>MELYRDPSQPIEVRVRDLLSRMTLEEKVAQLGSVWGYELIDERGKFSREKAKELLKNGIGQITRPGGSTNLEPQEAAELVNEIQRFLVEETRLGIPAMIHEECLTGYMGLGGTNFPQAIAMASTWDPDLIEKMTTAVREDMRKIGAHQGLAPVLDVARDPRWGRTEETFGESPYLVARMGVSYVKGLQGEDIKKGVVATVKHFAGYSASEGGKNWAPTNIPEREFKEVFLFPFEAAVKEANVLSVMNSYSEIDGVPCAANRKLLTDILRKDWGFEGIVVSDYFAVKVLEDYHRIARDKSEAARLALEAGIDVELPKTECYQYLKDLVEKGIISEALIDEAVTRVLRLKFMLGLFENPYVEVEKAKIESHRDIALEIARKSIILLKNDGILPLQKNKKVALIGPNAGEVRNLLGDYMYLAHIRALLDNIDDVFGNPQIPRENYERLKKSIEEHMKSIPSVLDAFKEEGIEFEYAKGCEVTGEDRSGFEEAIEIAKKSDVAIVVVGDKSGLTLDCTTGESRDMANLKLPGVQEELVLEVAKTGKPVVLVLITGRPYSLKNVVDKVNAILQVWLPGEAGGRAIVDIIYGKVNPSGKLPISFPRSAGQIPVFHYVKPSGGRSHWHGDYVDESTKPLFPFGHGLSYTKFEYSNLRIEPKEVPPAGEVVIK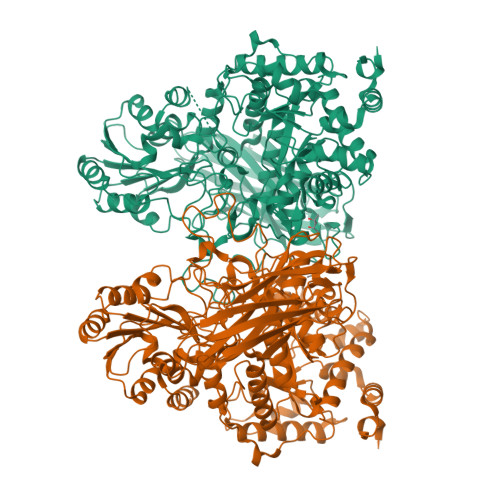VDVENIGDRDGDEVVQLYIGREFASVTRPVKELKGFKRVSLKAKEKKTVVFRLHMDVLAYYNRDMKLVVEPGEFKVMVGSSSEDIRLTGSFSVVGEKREVVGMRKFFTEACEEAAALEENLYFQGAHHHHHHHHHH[2x]> MPQYQTWEEFSRAAEKLYLADPMKARVVLKYRHSDGNLCV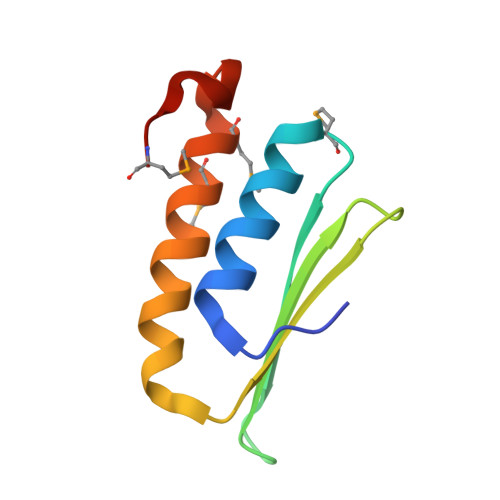KVTDDLVCLVYKTDQAQDVKKIEKFHSQLMRLMVAKEARNVTMET> MPYIVDVYAREVLDSRGNPTVEVEVYTETGAFGRALVPSGASTGEYEAVELRDGDKDRYLGKGVLTAVNNVNEIIAPELLGFDVTEQNAIDQLLIELDGTENKGKLGANAILGVSMACARAAADFLQIPLYQYLGGFNSKTLPVPMMNIVNGGEHADNNVDIQEFMIMPVGAPNFREALRMGAQIFHSLKSVLSAKGLNTAV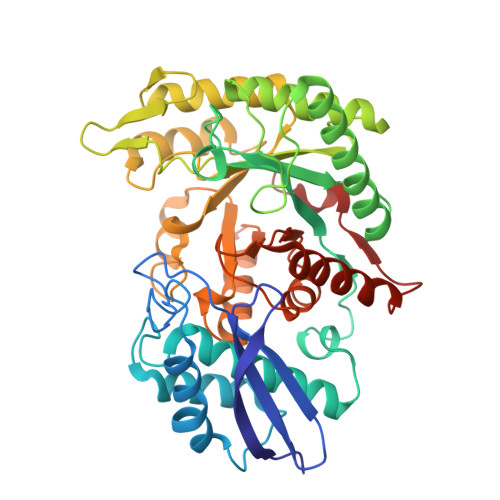GDEGGFAPNLGSNEEALQTIVEAIEKAGFKPGEEVKLAMDAASSEFYNKEDGKYHLSGEGVVKTSAEMVDWYEELVSKYPIISIEDGLDENDWEGHKLLTERLGKKVQLVGDDLFVTNTKKLSEGIKNGVGNSILIKVNQIGTLTETFDAIEMAKRAGYTAVISHRSGETEDSTIADIAVATNAGQIKTGAPSRTDRVAKYNQLLRIEDQLAETAQYHGINSFYNLNK> MAKNTDKAQLALGDHAARQLANATKTAPQLSTITPRWLTHLLQWIPVEAGIYRLNRVNNTDDIQVACTQRDEATLPQTFVDYAPEPREYFLNGVSTVLDVHTRVADLYSSPHDQIKEQLRLTIETIKERQESELINNPEYGLLASVTDDQRISTLNGPPTPDDLDDLLRKVWKEPGFFLAHPDAIAAFGRECTRRGVPPPTVSLFGSQFITWRGIPLIPSNKIPVEDGKTKILLLRVGEKRQGIVGLFQPGLAGEQSPGLSVRFMGINRNAIASYL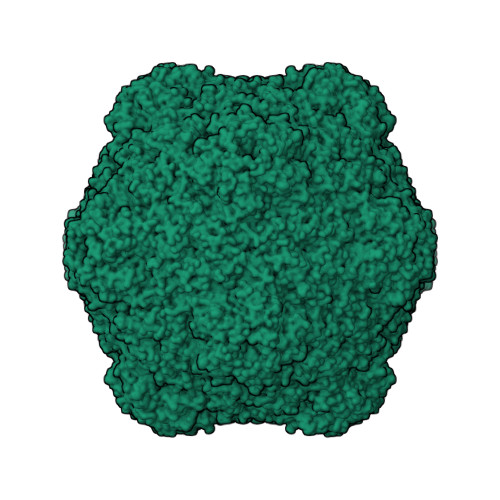ISLYCSLAVLTDDALAVLDDVEVDKYHDYPVNYK>[2x]MATSLNTIDIQGDILVGMHKQKQLFYFFAINDPATFKTHLASDIAPVVASVTQLSNVATQPLVALNIAFSNTGLLALGVTDNLGDSLFANGQAKDATSFKESTSSWVPQFAGTGIHGVIILASDTTDLIDQQVASIESTFGSSISKLYSLSASIR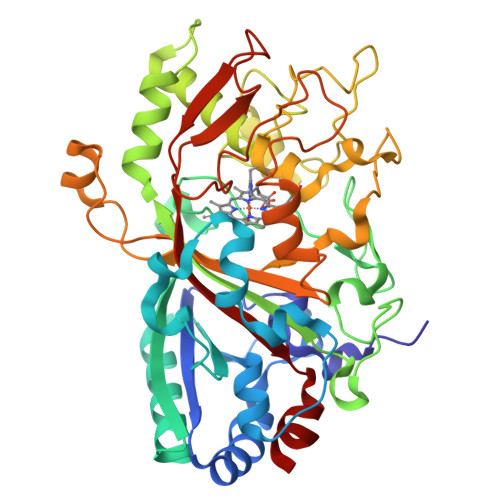PGNEAGHEMFGFLNGIAQPAINGFNTPLPGQNIVDAGVIITGATNDPITRPSWAVGGSFLAFRQLEQLVPEFNKYLLDNAPAGSGSLQARADLLGARMVGRWKSGAPIDLTPTADDPALGADAQRNNNFTYSHAGFDLGSDQSHCPFSAHIRKTRPRADLGGSLTPPNLSAGANSIMRSGIPYGPEVTSAESASNTTTQERGLAFVAYQAQLSQGFHFLQQTWADNANFPPGKTPATVGLDPIIGQNNGQPRVVNGLLPSNSSASLSIPQFVVSHGGEYFFSPPISAIGGRLSA phosphono hexadecanoate | C16 H33 O5 P 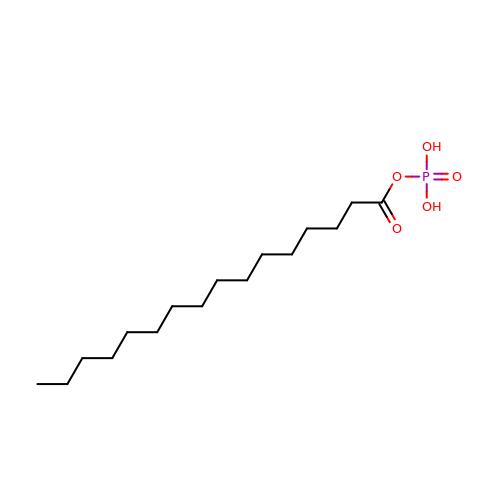| KUIJPSLAGAQZTC-UHFFFAOYSA-N> GPLSLSVDAFKILAAPKWEFPRKNLVLGKTLGEGEFGKVVKATAFHLKGRAGYTTVAVKMLKENASPSELRDLLSEFNVLKQVNHPHVIKLYGACSQDGPLLLIVEYAKYGSLRGFLRESRKVGPGPDERALTMGDLISFAWQISQGMQYLAEMKLVHRDLAARNILVAEGRKMKISDFGLSRDVYEEDFYVKRSQGRIPVKWMAIESLFDHIYTTQSDVWSFGVLLWEIVTLGGNPYPGIPPERLFNLLKTGHRMERPDNCSEEMYRL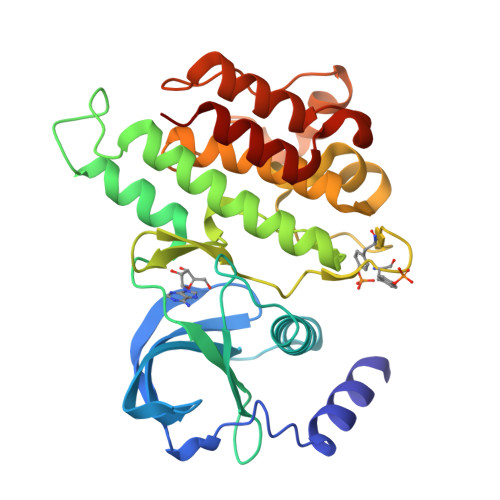MLQCWKQEPDKRPVFADISKDLEKMMVKRR>MAHHHHHHMSSKQFKILVNEDYQVNVPSLPIRDVLQEIKYCYRNGFEGYVFVPEYCRDLVDCDRKDHYVIGVLGNGVSDLKPVLLTEPSVMLQ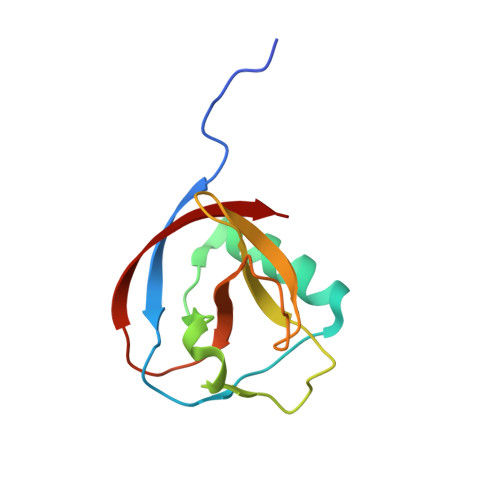GFIVRANCNGVLEDFDLKIA[2x]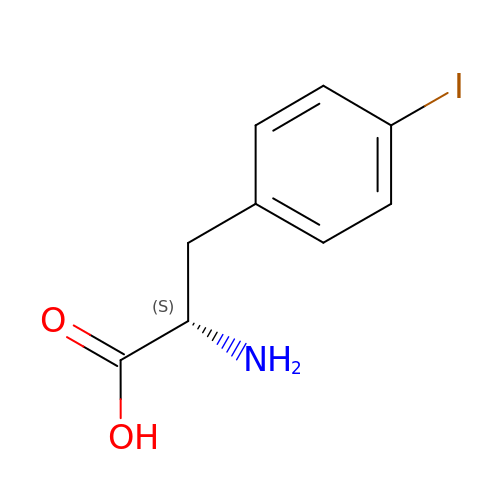IODO-PHENYLALANINE | C9 H10 I N O2 | PZNQZSRPDOEBMS-QMMMGPOBSA-N>MPIIGRKIQDKLNKTKDDISKNMSFLKVDKEYVKALPSQGLSSSAVLEKLKEYSSMDAFWQEGRASGTVYSGEEKLTELLVKAYGDFAWSNPLHPDIFPGLRKIEAEIVRIACSLFNGGPDSCGCVTSGGTESILMACKAYRDLAFEKGIKTPEIVAPQSAHAAFNKAASYFGMKIVRVPLTKMMEVDVRAMRRAISRNTAMLVCSTPQFPHGVIDPVPEVAKLAVKYKIPLHVDACLGGFLIVFMEKAGYPLEHPFDFRVKGVTSISADTHKYGYAPKGSSLVLYSDKKYRNYQFFVDTDWQGGIYASPTIAGSRPGGISAACWAALMHFGENGYVEATKQIIKTARFLKSELENIKGIFVFGNPQLSVIALGSRDFDIYRLSNLMTAKGWNLNQLQFPPSIHFCITLLHARKRVAIQFLKDIRESVTQIMKNPKAKTTGMGAIYGMAQTTVDRNMVAELSSVFLDSLYSTDTVTQGSQMNGSPKPHHHHHHH[2x]

Deacylation of Cer to sphingosine and subsequent phosphorylation by sphingosine kinase lead to the formation of sphingosine-1-phosphate (S1P), whose irreversible degradation by S1P lyase (SPL) terminates sphingolipid metabolism. SPL (EC 4.1.2.27) is a pyridoxal 5′-phosphate (PLP)-dependent enzyme bound to the endoplasmic reticulum membrane through an N-terminal sequence, with the catalytic domain facing the cytosol. The protein is a tight dimer and belongs to the Fold Type I family. The active site is formed by residues from both subunits and comprises an Y-shaped channel whose distal part is largely hydrophobic.

To confirm the soundness of our virtual screening campaign, we solved the crystal structures of unbound hSPL and AfuSPL at 1.8 Å and 3.5 Å resolution, respectively. The structure of ligand-free hSPL was superposable with the one solved in complex with a known active site inhibitor with a RMSD of 0.36 Å (between 443 Cα pairs), suggesting that hSPL does not undergo extensive conformational changes upon ligand binding. Access to the active site is guaranteed by a deep cleft flanked by the last two C-terminal helices. The surface of this cleft is highly hydrophobic to accommodate the aliphatic tail of S1P. Therefore, the rigidity of the hSPL structure may account for the need to prevent a hydrophobic collapse that would close the substrate binding site. PLP is bound through a Schiff base linkage with a lysine residue that in the human enzyme complexed with a known inhibitor is Lys359 (internal aldimine). In the visible region, hSPL shows an absorbance maximum centered at 426 nm and a shoulder at about 340 nm, attributable to the ketoenamine and enolimine tautomers of the internal aldimine, respectively. In agreement with SPL being a well conserved protein from bacteria to humans, we found that hSPL and AfuSPL show very similar biochemical properties, although we could notice differences related to (i) an higher propensity of the fungal enzyme to bind the hydrophobic probe ANS, which may also correlate with the higher aggregation tendency and reduced purification yields, and (ii) some changes in the spectral and kinetic features, probably due to subtle differences in the region surrounding the active site. In this regard, the crystal structures of the two proteins in the ligand-free form confirm that the coenzyme binding regions are superimposable, thus further supporting the possibility to develop a dual-species inhibitor. Indeed, when C17 was docked in the catalytic pocket of both hSPL and AfuSPL, the best predicted poses were in the entrance of the narrow and hydrophobic channel. In both enzymes, one of the aromatic thienyl rings of C17 stabilizes the binding by π-stacking with Phe545(A) and Phe565(A) of hSPL and AfuSPL, respectively.> MSRKQLALFEPTLVVQALKEAVKKLNPQAQWRNPVMFIVWIGSLLTTCISIAMASGAMPGNALFSAAISGWLWITVLFANFAEALAEGRSKAQANSLKGVKKTAFARKLREPKYGAAADKVPADQLRKGDIVLVEAGDIIPCDGEVIEGGASVDESAITGEAAPVIRESGGDFASVTGGTRILSDWLVIECSVNPGETFLDRMIAMVEGAQRRKTPNEIALTILLIALTIVFLLATATLWPFSAWGGNAVSVTVLVALLVCLIPTTIGGLLSAIGVAGMSRMLGANVIATSGRAVEAAGDVDVLLLDKTGTITLGNRQASEFIPAQGVDEKTLADAAQLASLADETPEGRSIVILAKQRFNLRERDVQSLHATFVPFTAQSRMSGINIDNRMIRKGSVDAIRRHVEANGGHFP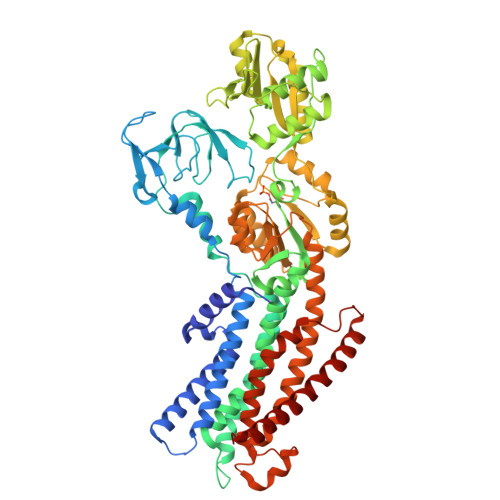TDVDQKVDQVARQGATPLVVVEGSRVLGVIALKDIVKGGIKERFAQLRKMGIKTVMITGDNRLTAAAIAAEAGVDDFLAEATPEAKLALIRQYQAEGRLVAMTGDGTNDAPALAQADVAVAMNSGTQAAKEAGNMVDLDSNPTKLIEVVHIGKQMLMTRGSLTTFSIANDVAKYFAIIPAAFAATYPQLNALNIMCLHSPDSAILSAVIFNALIIVFLIPLALKGVSYKPLTASAMLRRNLWIYGLGGLLVPFIGIKVIDLLLTVCGLV>AFEDELGAQPPLGFFDPFGMLSGDCTQERFDRLRYVEIKHGRIAQLAFLGQIVTRAGIHLPGSINYAGDSFDSFPNGVAALFGPNSIPTAGLVQIIAFIGVLECAFMRDVPGTGNEHVGDFRNGYIDFGWDSFDEETKLQKRAIELNNGRAAMMGILGLMVHEEIIPLGYDPDLPIIGHLQ[3x]

Diatoms are dominant marine algae and contribute around a quarter of global primary productivity, the success of which is largely attributed to their photosynthetic capacity aided by specific fucoxanthin chlorophyll-binding proteins (FCPs) to enhance the blue-green light absorption under water. One of the important factors responsible for the powerful vitality of diatoms is their extraordinary light-harvesting capacity, which is achieved by their unique antenna system, fucoxanthin (Fx) chlorophyll (Chl) c binding proteins (FCPs). Here, we solved the structures of a PSII-FCPII supercomplex and a trimeric FCP from C. meneghiniana by single particle analysis using cryo-EM, which revealed detailed structures of monomeric, dimeric and trimeric FCPs, as well as their binding to the PSII core. In conclusion, the cryo-EM structures of PSII-FCPII and the trimeric FCP of C. meneghiniana provide detailed insights into the structures of various FCP antennae and the assembly of FCPs within the PSII supercomplex.

The trimeric FCP of C. meneghiniana was determined as a homotrimer encoded by a gene homologous to fcp05 of C. cryptica. The molecule weight of Cm-FCP05 is around 19.7 kDa, consistent with the previous results. In each subunit of the Cm-FCP trimer, we assigned 8 Chls a, 3 Chls c, 7 Fxs and 1 sulfoquinovosyl diacylglycerol (SQDG) molecule. The secondary structure of Cm-FCP05 is similar to that of Pt-Lhcf4 and Cg-FCPII-A except for the existence of a longer C-terminal loop. Cm-FCP05 exhibits a unique “head-to-tail” assembly pattern due to its specific loops and lipids, forming enlarged spaces between each monomer to accommodate more Chls and carotenoids. An extra Chl a412 and an SQDG molecule are inserted into the gap between helices A and C at the lumenal surface, building hydrophobic interactions and hydrogen bonds with Chls c405, Fx306 and Thr118 of B-C loop. At the stromal side, one specific Chl a402-c403-a406 cluster is located in the inner side of the trimer to hold the energy equilibrium among three monomers, and another Chl a401-c408-a407 cluster in the exterior region is responsible for EET to the PSII core or other FCP antennae. The distances among Chls a406 in the Cm-FCP05 trimer are larger than those in the Pt-Lhcf dimer; for this reason, an extra Chl a415 was found in the Cm-FCP05 trimer which may play a role in enhancing the efficient EET between the adjacent monomers. The trimeric Cm-FCP05 structure revealed in this study represents the atomic structure of FCP trimer containing a substantial amount of red Fx and Chls c, enabling the capture of blue-green light. The Cm-FCP05 trimer found here may have weaker associations with the PSII core and detach into free FCPs, which are recovered on the top of SDG.> HHHHHHVIDELLLFWNLAETDRVLDELEEALLVSDFGPKITVRIVERLREDIMSGKLKSGSEIKDALKESVLEMLAKKNSKTELQLGFR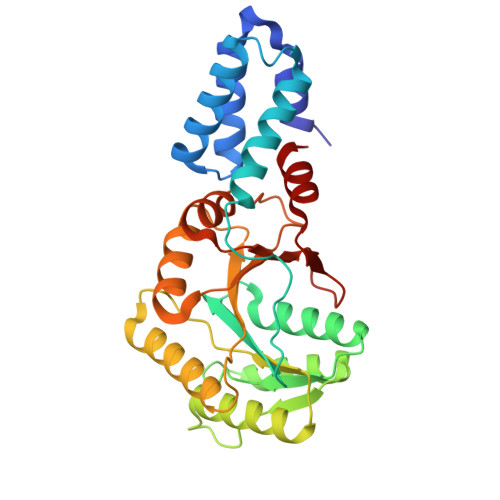KPAVIMIVGVNGGGKTTSLGKLAHRLKNEGTKVLMAAGDTFRAAASDQLEIWAERTGCEIVVAEGDKAKAATVLSKAVKRGKEEGYDVVLCDTSGRLHTNYSLMEELIACKKAVGKIVSGAPNEILLVLDGNTGLNMLPQAREFNEVVGITGLILTKLDGSARGGCVVSVVEELGIPVKFIGVGEAVEDLQPFDPEAFVNAIFS Botulinum neurotoxin A1 (BoNT/A1) belongs to the most potent toxins and is used as a major therapeutic agent. BoNTs and BoNT-like proteins share a common domain organization and are produced as precursors that are cleaved into a 50 kDa light chain (LC) and a 100 kDa heavy chain (HC) that with the exception of BoNT/Wo remain connected by a disulfide bond. The LC is a zinc metalloprotease that specifically cleaves soluble N-ethylmaleimide-sensitive-factor attachment receptor (SNARE) proteins. While the physiological functions of SV2 proteins remains to be determined, their best-established role is to act as receptors for several BoNTs (BoNT/A, /D, /E, and /F).

To obtain a more complete picture of toxin conformations, we set out to solve the structure of full-length BoNT/A1 by single-particle cryo-EM. Towards this goal, an inactive variant was recombinantly produced in E. coli and purified to homogeneity. Particle sizes obtained for BoNT/A1 were consistent with the presence of a monomer. The best subset of particles yielded a cryo-EM density at an overall resolution of 3.8 Å. Based on our 2D and 3D classification, the semi-closed toxin state is the dominant species, although BoNT/A1 appears to sample a wide range of HC domain orientations in solution, including the open conformation. The HC density in our best 3D class for the BoNT/A1 in solution is relatively poorly defined, which reflects the previously reported high mobility of the HC. The poor density allowed only manual rigid-body docking of the domain into the semi-closed orientation. Key elements of the HN domain that have been previously suggested to play an important role in toxin translocation, such as the switch region (E620-F667)32 and most of the belt (N493-D546) are relatively well resolved despite the moderate overall resolution of the cryo-EM map (we omitted the first two residues of the belt due to weak density). The conformation of BoNT/A1 seen in the cryo-EM structure markedly differs from the open conformation observed in the X-ray crystal structure. Superimposition of the cryo-EM and the X-ray crystal structure of BoNT/A1 demonstrates that the LC and the HN domain arrangement is very similar and that the two structures basically differ by a ~ 107° rotation of the HC domain. The state of BoNT/A1 in solution captured by cryo-EM is reminiscent of the semi-open conformation of the closely-related tetanus toxin at pH 5.5–6.5.

> MRGSHHHHHHGSLVPRGSPFVNKQFNYKDPVNGVDIAYIKIPNAGQMQPVKAFKIHNKIWVIPERDTFTNPEEGDLNPPPEAKQVPVSYYDSTYLSTDNEKDNYLKGVTKLFERIYSTDLGRMLLTSIVRGIPFWGGSTIDTELKVIDTNCINVIQPDGSYRSEELNLVIIGPSADIIQFECKSFGHEVLNLTRNGYGSTQYIRFSPDFTFGFEESLEVDTNPLLGAGKFATDPAVTLAHQLIHAGHRLYGIAINPNRVFKVNTNAYYEMSGLEVSFEELRTFGGHDAKFIDSLQENEFRLYYYNKFKDIASTLNKAKSIVGTTASLQYMKNVFKEKYLLSEDTSGKFSVDKLKFDKLYKMLTEIYTEDNFVKFFKVLNAKTFLNFDKAVFKINIVPKVNYTIYDGFNLRNTNLAANFNGQNTEINNMNFTKLKNFTGLFEFYKLLCVRGIITSKTKSLDKGYNKALNDLCIKVNNWDLFFSPSEDNFTNDLNKGEEITSDTNIEAAEENISLDLIQQYYLTFNFDNEPENISIENLSSDIIGQLELMPNIERFPNGKKYELDKYTMFHYLRAQEFEHGKSRIALTNSVNEALLNPSRVYTFFSSDYVKKVNKATEAAMFLGWVEQLVYDFTDETSEVSTTDKIADITIIIPYIGPALNIGNMLYKDDFVGALIFSGAVILLEFIPEIAIPVLGTFALVSYIANKVLTVQTIDNALSKRNEKWDEVYKYIVTNWLAKVNTQIDLIRKKMKEALENQAEATKAIINYQYNQYTEEEKNNINFNIDDLSSKLNESINKAMININKFLNQCSVSYLMNSMIPYGVKRLEDFDASLKDALLKYIYDNRGTLIGQVDRLKDKVNNTLSTDIPFQLSKYVDNQRLLSTFTEYIKNIINTSILNLRYESNHLIDLSRYASKINIGSKVNFDPIDKNQIQLFNLESSKIEVILKNAIVYNSMYENFSTSFWIRIPKYFNSISLNNEYTIINCMENNSGWKVSLNYGEIIWTLQDTQEIKQRVVFKYSQMINISDYINRWIFVTITNNRLNNSKIYINGRLIDQKPISNLGNIHASNNIMFKLDGCRDTHRYIWIKYFNLFDKELNEKEIKDLYDNQSNSGILKDFWGDYLQYDKPYYMLNLYDPNKYVDVNNVGIRGYMYLKGPRGSVMTTNIYLNSSLYRGAKFIIKKYASGNKDNIVRNNDRVYINVVVKNKEYRLATNASQAGVEKILSALEIPDVGNLSQVVVMKSKNDQGITNKCKMNLQDNNGNDIGFIGFHQFNNIAKLVASNWYNRQIERSSRTLGCSWEFIPVDDGWGERPLVPPTPGSAWSHPQFEK>[10x]TPQNITDLCAEYHNTQIHTLNDKIFSYTESLAGKR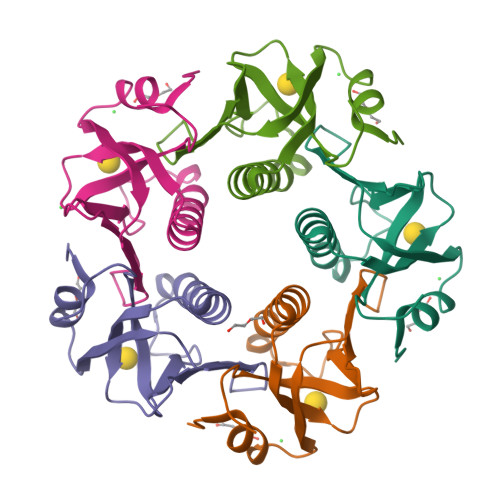EMAIITFKNGATFQVEVPGSQHIDSQKKAIERMKDTLRIAYLTEAKVEKLCVWNNKTPHAIAAISMANDKKIEYNETWYSRD>[2x]SERFPNDVDPIETRDWLQAIESVIREEGVERAQYLIDQLLAEARKGGVNVAAGTGISNYINTIPVEEQPEYPGNLELERRIRSAIRWNAIMTVLRASKKDLELGGHMASFQSSATIYDVCF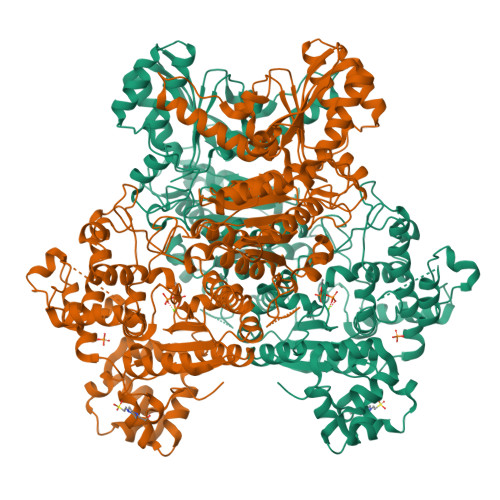NHFFRARNEQDGGDLVYFQGHISPGVYARAFLEGRLTQEQLDNFRQEVHGNGLSSYPHPKLMPEFWQFPTVSMGLGPIGAIYQAKFLKYLEHRGLKDTSKQTVYAFLGDGEMDEPESKGAITIATREKLDNLVFVINCNLQRLDGPVTGNGKIINELEGIFEGAGWNVIKVMWGSRWDELLRKDTSGKLIQLMNETVDGDYQTFKSKDGAYVREHFFGKYPETAALVADWTDEQIWALNRGGHDPKKIYAAFKKAQETKGKATVILAHTIKGYGMGDAAEGKNIAHQVKKMNMDGVRHIRDRFNVPVSDADIEKLPYITFPEGSEEHTYLHAQRQKLHGYLPSRQPNFTEKLELPSLQDFGALLEEQSKEISTTIAFVRALNVMLKNKSIKDRLVPIIADEARTFGMEGLFRQIGIYSPNGQQYTPQDREQVAYYKEDEKGQILQEGINALGAGCSWLAAATSYSTNNLPMIPFYIYYSMFGFQRIGDLCWAAGDQQARGFLIGGTSGRTTLNGEGLQHEDGHSHIQSLTIPNCISYDPAYAYEVAVIMHDGLERMYGEKQENVYYYITTLNENYHMPAMPEGAEEGIRKGIYKLETIEGSKGKVQLLGSGSILRHVREAAEILAKDYGVGSDVYSVTSFTELARDGQDCERWNMLHPLETPRVPYIAQVMNDAPAVASTDYMKLFAEQVRTYVPADDYRVLGTDGFGRSDSRENLRHHFEVDASYVVVAALGELAKRGEIDKKVVADAIAKFNIDADKVNPRLA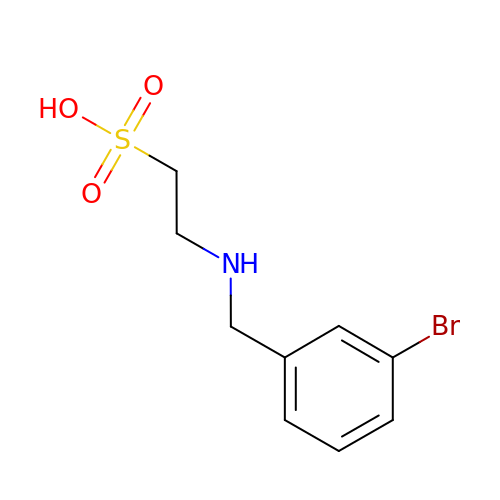2-[(3-bromobenzyl)amino]ethanesulfonic acid | C9 H12 Br N O3 S | ZPPIYSKMLNAVOI-UHFFFAOYSA-N> 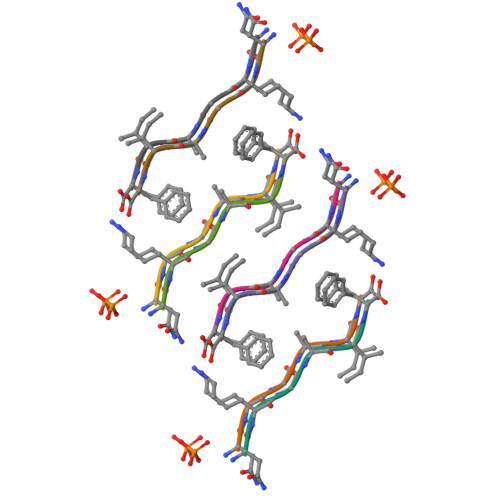NKGAIF>[12x]MSKPQPIAAANWKCNGSQQSLSELIDLFNSTSINHDVQCVVASTFVHLAMTKERLSHPKFVIAAQNAIAKSGAFTGE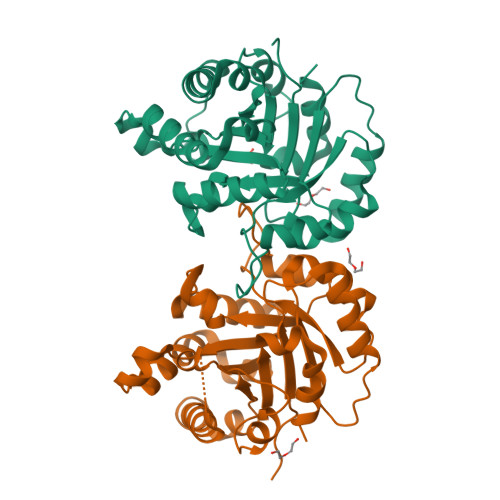VSLPILKDFGVNWIVLGHSERRAYYGDTNEIVADKVAAAVASGFMVIACIGETLQERESGRTAVVVLTQIAAIAKKLKKADWAKVVIAYEPVWAIGTGKVATPQQAQEAHALIRSWVSSKIGADVAGELRILYGGSVNGKNARTLYQQRDVNGFLVGGASLKPEFVDIIKATQ>[2x]SERFPNDVDPIETRDWLQAIESVIREEGVERAQYLIDQLLAEARKGGVNVAAGTGISNYINTIPVEEQPEYPGNLELERRIRSAIRWNAIMTVLRASKKDLELGGHMAS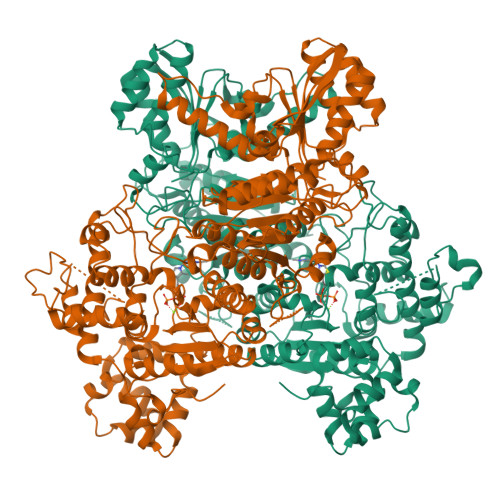FQSSATIYDVCFNHFFRARNEQDGGDLVYFQGHISPGVYARAFLEGRLTQEQLDNFRQEVHGNGLSSYPHPKLMPEFWQFPTVSMGLGPIGAIYQAKFLKYLEHRGLKDTSKQTVYAFLGDGEMDEPESKGAITIATREKLDNLVFVINCNLQRLDGPVTGNGKIINELEGIFEGAGWNVIKVMWGSRWDELLRKDTSGKLIQLMNETVDGDYQTFKSKDGAYVREHFFGKYPETAALVADWTDEQIWALNRGGHDPKKIYAAFKKAQETKGKATVILAHTIKGYGMGDAAEGKNIAHQVKKMNMDGVRHIRDRFNVPVSDADIEKLPYITFPEGSEEHTYLHAQRQKLHGYLPSRQPNFTEKLELPSLQDFGALLEEQSKEISTTIAFVRALNVMLKNKSIKDRLVPIIADEARTFGMEGLFRQIGIYSPNGQQYTPQDREQVAYYKEDEKGQILQEGINELGAGCSWLAAATSYSTNNLPMIPFYIYYSMFGFQRIGDLCWAAGDQQARGFLIGGTSGRTTLNGEGLQHEDGHSHIQSLTIPNCISYDPAYAYEVAVIMHDGLERMYGEKQENVYYYITTLNENYHMPAMPEGAEEGIRKGIYKLETIEGSKGKVQLLGSGSILRHVREAAEILAKDYGVGSDVYSVTSFTELARDGQDCERWNMLHPLETPRVPYIAQVMNDAPAVASTDYMKLFAEQVRTYVPADDYRVLGTDGFGRSDSRENLRHHFEVDASYVVVAALGELAKRGEIDKKVVADAIAKFNIDADKVNPRLA>[4x]MGRKKIQISRILDQRNRQVTFTKRKFGLMKKAYELSVLCDCEIALIIFNSANRLFQYASTDMDRVLLKYTEYSEPHESRTNTDILETLKRRGI;>SP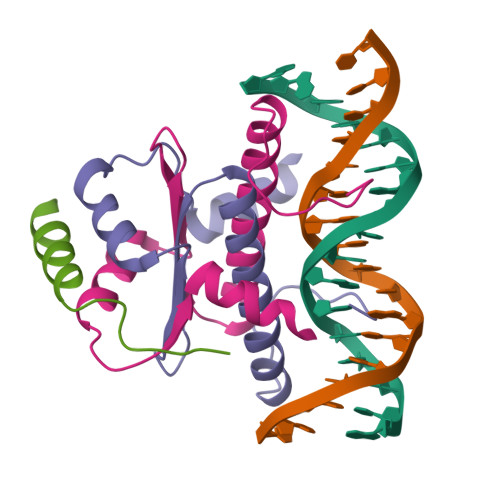KGTGASTEVKQKLQEFLLSKSATK[2x]>RRWTFVRYHYINKAYEVTMKIQIISGFDRQLTAWLRVHGRRLTNNQKKTLFFVNRRYMQTHWQNYMLWVKRKIKALGRPAAVGDYTRLGAEIGRRVDMVFFYNFLSGRKMIPPYSAYMAKLNALRPADVPVKNHGK[2x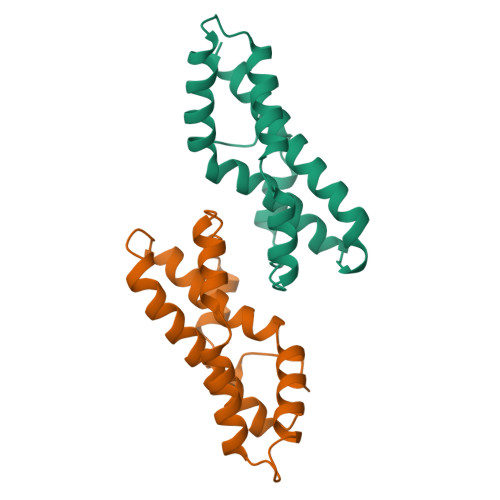]> MHHHHHHSSGRENLYFQGGGYEIPARLRTLHNLVIQYASQG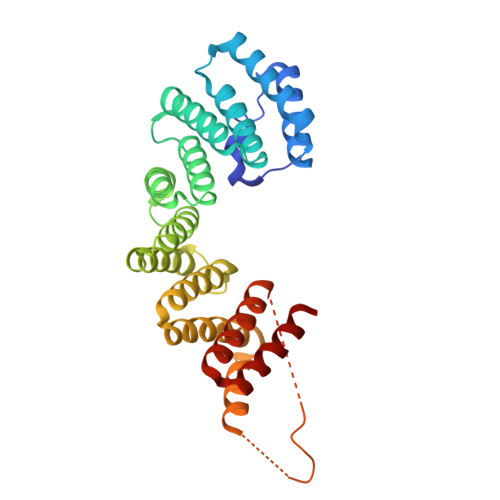RYEVAVPLCKQALEDLEKTSGHDHPDVATMLNILALVYRDQNKYKDAANLLNDALAIREKTLGKDHPAVAATLNNLAVLYGKRGKYKEAEPLCKRALEIREKVLGKDHPDVAKQLNNLALLCQNQGKYEEVEYYYQRALEIYQTKLGPDDPNVAKTKNNLASCYLKQGKFKQAETLYKEILTRAHEREFGSVDDENKPIWMHAEEREECKGKQKDGTSFGEYGGWYKACKVDSPTVTTTLKNLGALYRRQGKFEAAETLEEAAMRSRKQG7-cyclohexylheptyl 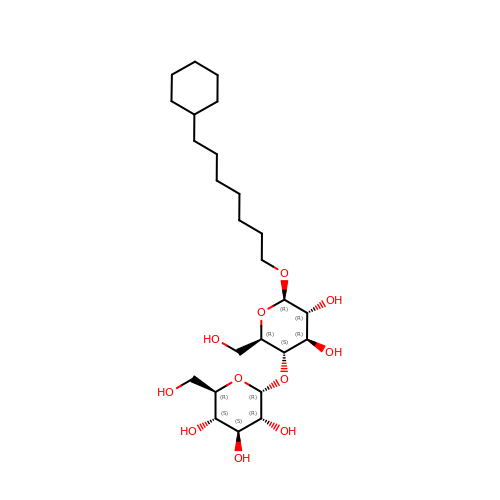4-O-alpha-D-glucopyranosyl-beta-D-glucopyranoside | C25 H46 O11 | BEKAVONQUWHNMM-IYBATYGCSA-N>MHHHHHHMANRKLEKMASIDVHLRQLVPGKVSEDDKLVEYDALLLDRFLDILQDLHGEDLRETVQELYEHSAEYEGKHEPKKLEELGSVLTSLDPGDSIVIAKAFSHMLNLANLAEEVQIAYRRRIKKLKKGDFVDESSATTESDLEETFKKLVGDLNKSPEEIFDALKNQTVDLVLTAHPTQSVRRSLLQKHGRIRDCLAQLYAKDITPDDKQELDEALQREIQAAFRTDEIKRTPPTPQDEMRAGMSYFHETIWKGVPKFLRRVDTALKNIGIEERVPYNAPLIQFSSWMGGDRDGNPRVTPEVTRDVCLLARMMAATMYFNQIEDLMFEMSMWRCNDELRARADEVHANSRKDAAKHYIEFWKSIPTTEPYRVILGDVRDKLYHTRERAHQLLSNGHSDVPVEATFINLEQFLEPLELCYRSLCSCGDRPIADGSLLDFLRQVSTFGLSLVRLDIRQESDRHTDVLDAITTHLDIGSYREWSEERRQEWLLSELSGKRPLFGSDLPKTEEIADVLDTFHVIAELPADSFGAYIISMATAPSDVLAVELLQRECRVKQPLRVVPLFEKLADLEAAPAAVARLFSVDWYKNRINGKQEVMIGYSDSGKDAGRLSAAWQLYKAQEELVKVAKEYGVKLTMFHGRGGTVGRGGGPTHLAILSQPPDTINGSLRVTVQGEVIEQSFGEEHLCFRTLQRFTAATLEHGMRPPISPKPEWRALLDEMAVVATEEYRSVVFQEPRFVEYFRLATPELEYGRMNIGSRPSKRKPSGGIESLRAIPWIFAWTQTRFHLPVWLGFGSAIRHVIEKDVRNLHMLQDMYQHWPFFRVTIDLIEMVFAK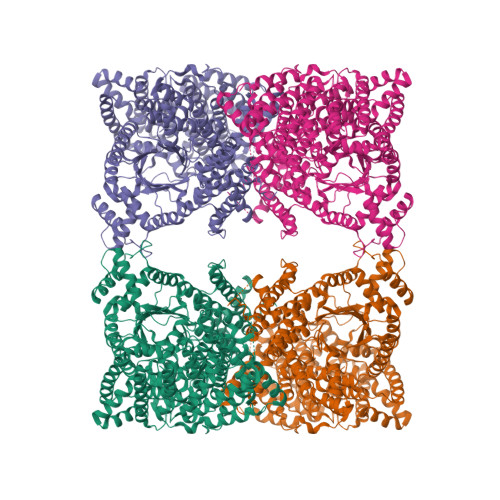GDPGIAALYDKLLVSEELWPFGEKLRANFEETKKLILQTAGHKDLLEGDPYLKQRLRLRDSYITTLNVCQAYTLKRIRDPSYHVTLRPHISKEIAESSKPAKELIELNPTSEYAPGLEDTLILTMKGIAAGLQNTG[3x]>MSAAEEIHTPRPAHVPADRVVELDMYNPQGIEKGYLEAWTSLQTADLPSMVWTPLNGGHWIATRGELIQDIYCDPDHFSSHVIFIPKAAGEKYAMVPSKMDPPEHRPYREVVDKGLNLRAIREREPAVRAHAIALIEAFADKGHCDFVEEFSGEFPIRVFMMMADLPMEDSPKLRAFAAGMTRPEGNTPTEMADALDRANRSFFDYVSPIIDARMGGDGTDILTLSINSQVNGAPMEREKLLGMVSLLLLAGLDTVTNFLNMTMDYLGRHPDKVRELTENPTEIRRGVEELFRRFPLVAAARMVAHDVERDGVELKQGEMVLLPTALHGLDPRVNADPWEVDFQRKRPAHSTFGNGPHRCAGLHLARLETTVMLEEWLKRIPTFRVVPGTGPTYHSGVV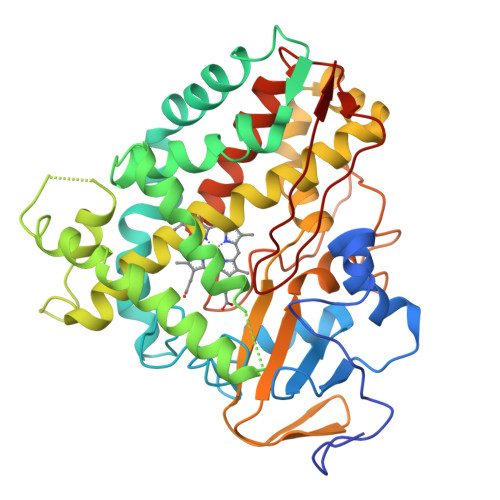ASVDGVRLEW[2x]> MEPFGTDERNWTHEEKDIITRFLKYDKHVNLKTAEMVYSAEVESAYFGKA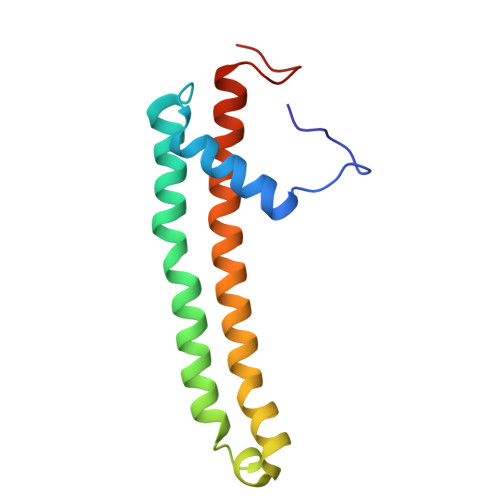GALAGGVISALFFNFPIVRNLPIIRRSVIGVLPFLYCYTWGKNTQEELRWLKTFAAYQRFVVYHGQHCKLWV>MTYTTRQIGAKNTLEYKVYIEKDGKPVSAFHDIPLYADKENNIFNMVVEIPRWTNAKLEITKEETLNPIIQDTKKGKLKFVRNCFPHHGYIHNYGAFPQTWEDPNVSHPETKAVGDNDPIDVLEIGETIAYTGQVKQVKALGIMALLDEGETDWKVIAIDINDPLAPKLNDIEDVEKYFPGLLRATNEWFRIYKIPDGKPENQFAFSGEAKNKKYALDIIKETHDSWKQLIAGKSSDSKGIDLTNVTLPDTPTYSKAASDAIPPASLKADAPIDKSIDKWFFISGSV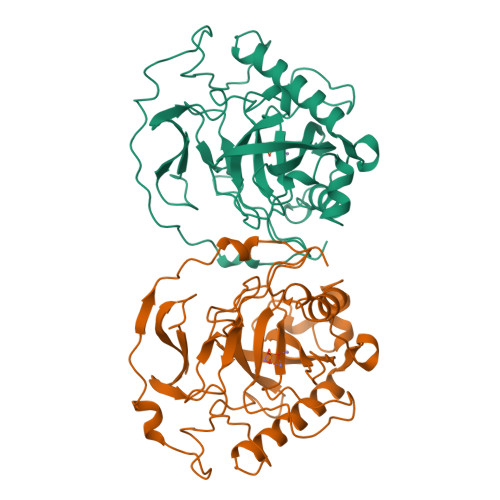[2x]> MGSDKIHHHHHHMRKVVKIAVILPMTGGISAFGRMVWEGIQIAHEEKPTVLGEEVELVLLDTRSEKTEAANAAARAIDKEKVLAIIGEVASAHSLAIAPIAEENKVPMVTPASTNPLVTQGRKFVSRVCFIDPFQGAAMAVFAYKNLGAKRVVVFTDVEQ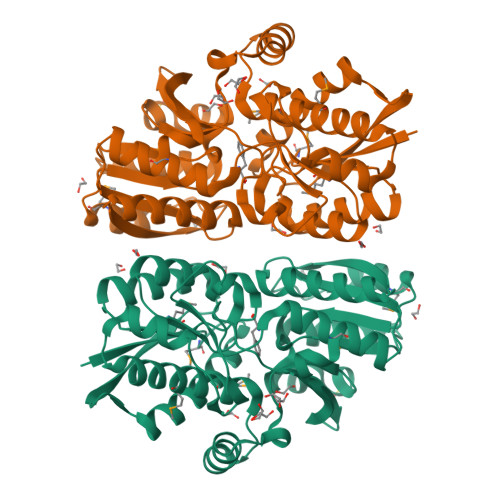DYSVGLSNFFINKFTELGGQVKRVFFRSGDQDFSAQLSVAMSFNPDAIYITGYYPEIALISRQARQLGFTGYILAGDGADAPELIEIGGEAVEGLLFTTHYHPKAASNPVAKKFVEVYKEKYGKEPAALNALGYDAYMVLLDAIERAGSFDREKIAEEIRKTRNFNGASGIINIDENGDAIKSVVVNIVKNGSVDFEAVINPDDLK> SMTEEERSSALSEVSLRLLCHDDIDTVKHLCGDWFPIEYPDSWYRDITSNKKFFSLAATYRGAIVGMIVAEIKNRTKIHKED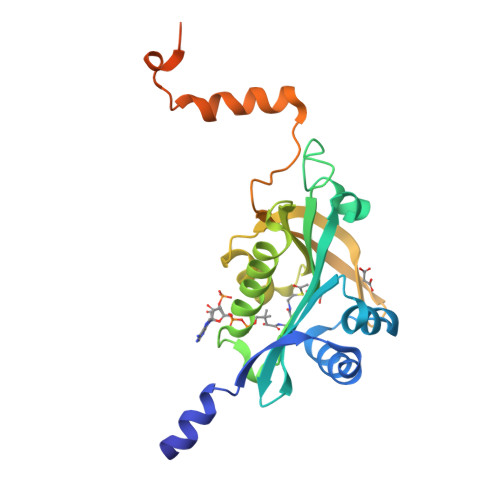GDILASNFSVDTQVAYILSLGVVKEFRKHGIGSLLLESLKDHISTTAQDHCKAIYLHVLTTNNTAINFYENRDFKQHHYLPYYYSIRGVLKDGFTYVLYINGGHPPWTILDYIQHLGSALASLSPCSIPHRVYRQAHSLLCSFLPWSGISSKSGIEYSRTM> MRSHTITMTTTSVSSWPYSSHRMRFITNHSDQPPQNFSATPNVTTCPMDEKLLSTVLTTSYSVIFIVGLVGNIIALYVFLGIHRKRNSIQIYLLNVAIADLLLIFCLPFRIMYHINQNKWTLGVILCKVVGTLFYMNMYISIILLGFISLDRYIKINRSIQQRKAITTKQSIYVCCIVWMLALGGFLTMIILTLKKGGHNSTMCFHYRDKHNAKGEAIFNFILVVMFWLIFLLIILSYIKIGKNLLRISKRGIDCSFWNESYLTGSRDERKKSLLSKFGMDEGVTFMFIGRFDRGQKGVDVLLKAIEILSSKKEFQEMRFIIIGKGDPELEGWARSLEEKHGNVKVITEMLSREFVRELYGSVDFVIIPSYFEPFGLVALEAMCLGAIPIASAVGGLRDIITNETGILVKAGDPGELA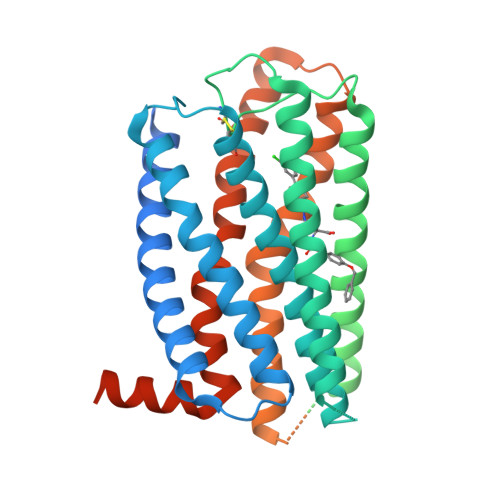NAILKALELSRSDLSKFRENCKKRAMSFSDQARMDIRLAKGKYATTARNSFIVLIIFTICFVPYHAFRFIYISSQLNVSSCYWKEIVHKTNEIMLVLSSFNSCLDPVMYFLMSSNIRKIMCQLLFRRFQGEPSRSESTSEFKPGYSLHDTSVAVKIQSSSKST>[6x]MAESPIGVVVSSRRNGPWAELTLVLTPQELDQGKRLLLGELVRVSSGGKDYVGMVLDGYYEPVGRSDPTYTLALAHINQVDLEKEDPWARKEVNFYHHRIVLLGRVVQGGLFAPSTRLLPPVVEARVYRMTEEELQRLLAAEVRTSGSVKAEGKRRYAFGHLAYGLEEGGEYPEVVKEVDPALFVGRRTANF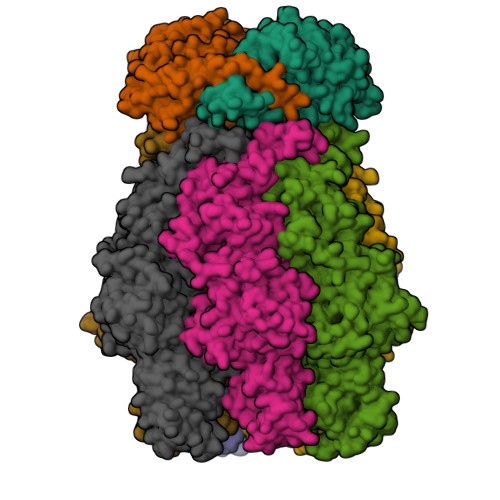GKTGFGKSNENKVILTLLAHAFPRVGMLILDQNAEYLLQTEATTSPGLAQAFKALGIRGRIRFYTAREEAWARRLKEHLGTEWREYVEVLPLKVDFYHFPELAVALAYQRRRLQGAEPPQYLENAFYNLEDWKHIPDRMAYVYGALRKAGLTPRKGLKIKYKNENYDISEEKSWGNLQEAMENNSQRGDNKGGARELYSRAKVFSFLRAFHAPGKEANFLETIKEDLLGEKTEGEGKVVILDLPSLGEAADFFTLRLMDLLFDRAVELYGKRQANFLVVLEEAHNFLEDKAGIFYRVAKEGRKYGIGMLYSTQSPASIPMEILSQTENFLVKHLSSEEDVKVLKRAKAPFAFVADFLLSEPIIGYSYVYFEPYQPFVVPLRVKLLEHVLKSLDS;>MPYAGEGSNPLGLKDFLDDLRLDHYQDLLRELDELYQKLKQERQVPLHGDGEAYPLLTLTVDGGEGRAFEELPLLSFGLVRVAAVGVKGFRLPSIAHLLPGYEVLRDPKGYLEGLLERSEESPAADALKTFFRATGISLEDLGEYYTKDLRAFMGIFRDVLEWAYLVWGVEKVLQESYKDYLFIKDGRLAQLGVRESFRSKLQNYFARKHLLLAGVTKRSRLLAEGLTSLVMARLFAEARGTFVLQVPQELMEKAYRYERQWNADLEGAFVMGRRYVARLLEDTFRPQEGVAIFDLPPYLGEEDAVKVARSLRAHRSVLYGGSVGTVVEAHGRASVARSIPRRMEEEILARFRKAFGEDLAKKLTEWLRLADRED[2x]>[24x]MSSQIRQNYSTEVEAAVNRLVNLYLRASYTYLSLGFYFDRDDVALEGVCHFFRELAEEKREGAERLLK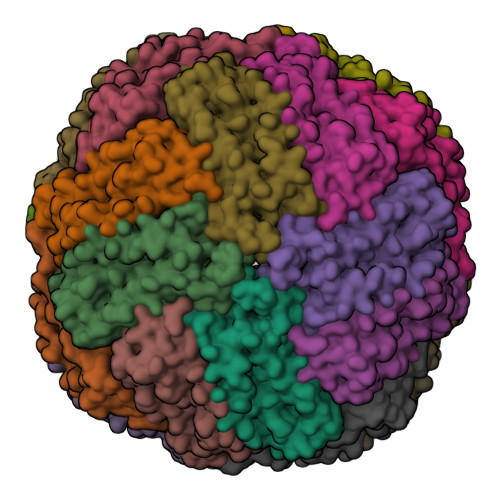MQNQRGGRALFQDLQKPSQDEWGTTLDAMKAAIVLEKSLNQALLDLHALGSAQADPHLCDFLESHFLDEEVKLIKKMGDHLTNIQRLVGSQAGLGEYLFERLTLKHD> GIQGLAKLIADVAPSAIRENDIKSYFGRKVAIDASMSIYQFLIAVRQGGDVLQNEEGETTSHLMGMFYRTIRMMENGIKPVYVFDGKPPQLKSGELAKASERRAEAEKQLQQAQAAGAEQEVEKFTKRLVKVTKQHNDECKHLLSLMGIPYLDAPSEAEASCAALVKAGKVYAAATEDMDCLTFGSPVLMRHLTASEAKKLPIQEFHLSRILQELGLNQEQFVDLCILLGSDYCESIRGIGPKRAVDLIQKHKSIEEIVRRLDPNKYPVPENWLHKEAHQLFLEPEVL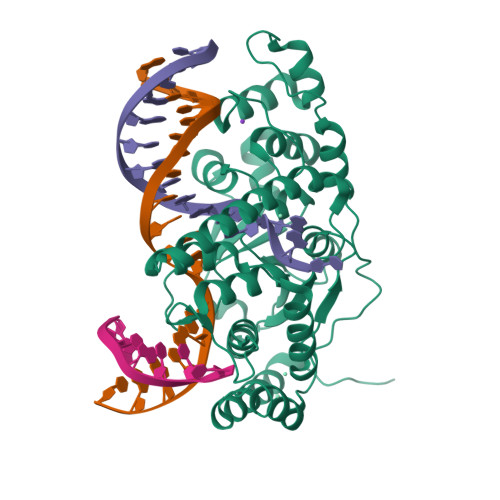DPESVELKWSEPNEEELIKFMCGEKQFSEERIRSGVKRLSKSRQGSTLEVLFQ> MMEGVRRAVAKFLRGGGVYEKAVDAFVKDLQRELIKADVNVKLVLNVTRRIKERALKEEPPPGVTRRDWMIKIVYEELVKLFGGDQEPQVDPPKTPWIVLLVGVQGSGKTTTAGKLAYYYVRRGYKVGLVSSDTHRPGAYEQLKRLAEEAGAMFYGEREGDPAEIARRGLEDLLSRGAEIVIVDTAGRHGHGEEARLLDEMKAIASKVRPDEVALVIDASI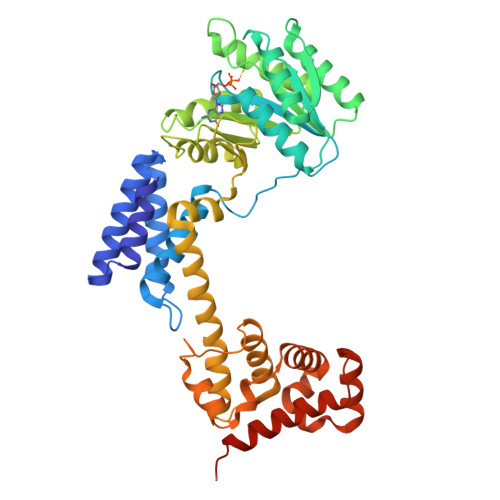GQKAMGLAERFHKSTPIGSIIVTKMDGTARGGGALTAAAVTGARIKFIGTGETLGELEPFAPRRFVARILGMGDLESLLERIKSLEEAGELDRAAEDVLKGRITMRTIYRQLRAMRKLGPLGKVLQMLPGASMLASIDEGALKLGEEKMKRWMAIIESMTYEELDRPEIIDKRRMRRIAIGSGTSVDDVRELLVYYKNLKTMMKKLKRDKRLLRRLGMEL>GPGSGTMLPVFCVVEHYENAIEYDCKEEHAEFVLVRKDMLFNQLIEMALLSLGYSHSSAAQAKGLIQVGKWNPVPLSYVTDAPDATVADMLQDVYHVVTLKIQLHSCPKLEDLPPEQWSHTTVRNALKDLLKDMNQSSLAKECPLSQSMISSIVNSTYYANVSAAKC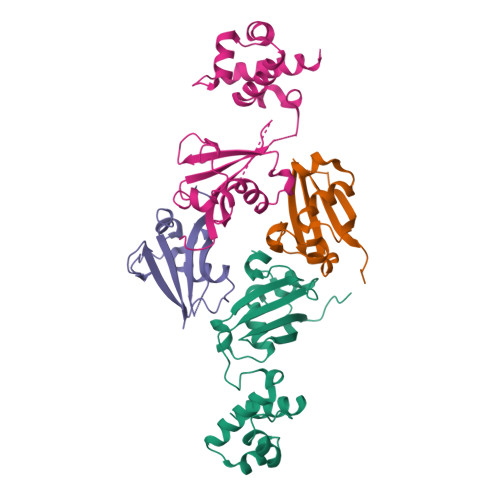QEFGRWYKHFKKT[4x]>[4x]MTPYEDLLRFVLETGTPKSDRTGTGTRSLFGQQMRYDLSAGFPLLTTKKVHFKSVAYELLWFLRGDSNIGWLHEHGVTIWDEWASDTGELGPIYGVQWRSWPAPSGEHIDQISAALDLLRTDPDSRRIIVSAWNVGEIERMALPPCHAFFQFYVADGRLSCQLYQRS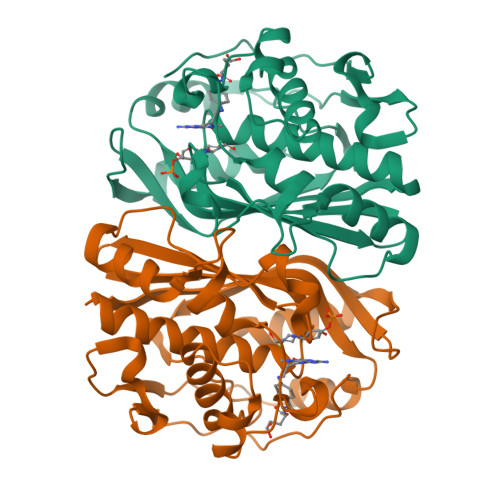ADLFLGVPFNIASYALLTHMMAAQAGLSVGEFIWTGGDCHIYDNHVEQVRLQLSREPRPYPKLLLADRDSIFEYTYEDIVVKNYDPHPAIKAPVAV>[4x]MAVTKLGINGFGRIGRLVFRAAFGRKDIEVVAINDPFMDLNHLCYLLKYDSVHGQFPCEVTHADGFLLIGEKKVSVFAEKDPSQIPWGKCQVDVVCESTGVFLTKELASSHLKGGAKKVIMSAPPKDDTPIYVMGINHHQYDTKQLIVSNASCTTNCLAPLAKVINDRFGIVEGLMTTVHASTANQLVVDGPSKGGKDWRAGRCALSNIIPASTGAAKAVGKVLPELNGKLTG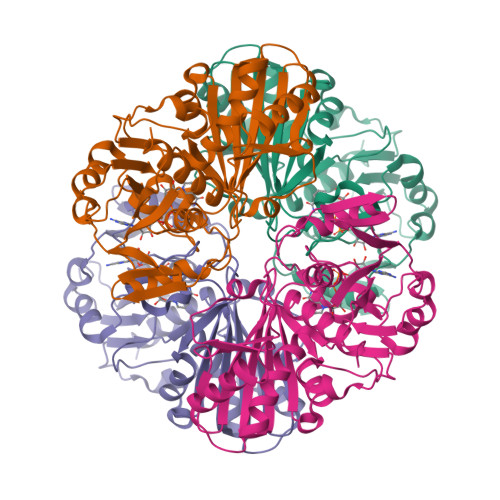VAFRVPIGTVSVVDLVCRLQKPAKYEEVALEIKKAAEGPLKGILGYTEDEVVSQDFVHDNRSSIFDMKAGLALNDNFFKLVSWYDNEWGYSNRVLDLAVHITNN> GLSAEQIAVPQEQGFELRDEGWEFGMSSKVLFGNNLDRLNPDSRNTLTKIARALLAVDIDKVRLEGHTDNYGDE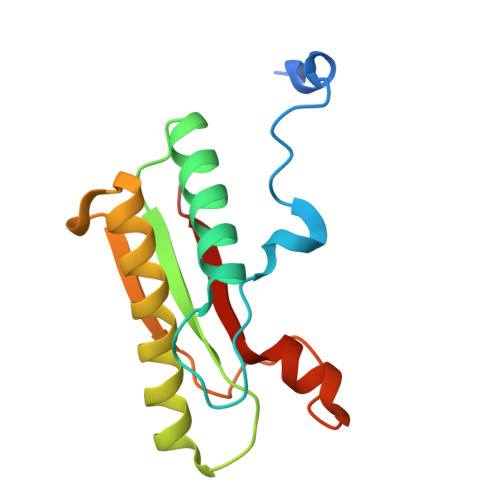GYNQKLSERRAESVAAVFREAGMPAANIEVRGLGMSKPVADNKTRAGRSENRRVAIIVPAE> MIIIRYLVRETLKSQLAILFILLLIFFCQKLVRILGAAVDGDIPANLVLSLLGLGVPEMAQLILPLSLFLGLLMTLGKLYTESEITVMHACGLSKAVLVKAAMILAVFTAIVAAVNVMWAGPWSSRHQDEVLEEAKANPGMAALAQGQFQQATNGS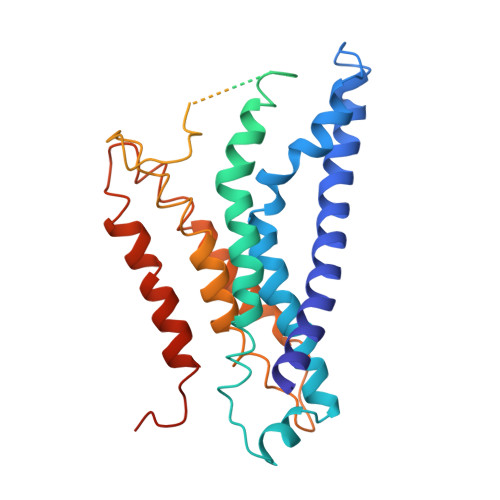SVLFIESVDGSDFKDVFLAQIRPKGNARPSVVVADSGHLTQLRDGSQVVTLNQGTRFEGTALLRDFRITDFQDYQAIIGHQAVALDPNDTDQMDMRTLWNTDTDRARAELNWRITLVVTVFMMALMVVPLSVVNPRQGRVLSMLPAMLLYLLFFLIQTSLKSNGGKGKLDPTLWMWTVNLIYLALAIVLNLWDTVFVRRLRASFSRKGAV>MPLIFKIGYNVIPLQDVILPTPSSKVLKYLIQSGKLIPSLKDLITSRDKYKPIFISHLGFNQRRIFQTNGNLKTITKGSRLSSIIAFSTQANVLSEVADEGIFETVYGKFHIMIESIEIVEVEKLKEEVEKHMNDNIRVRFVSPTLLSSKVLLPPSLSERYKKIHAGYSTLPSVGLIVAYAYNVYCNLIGKKE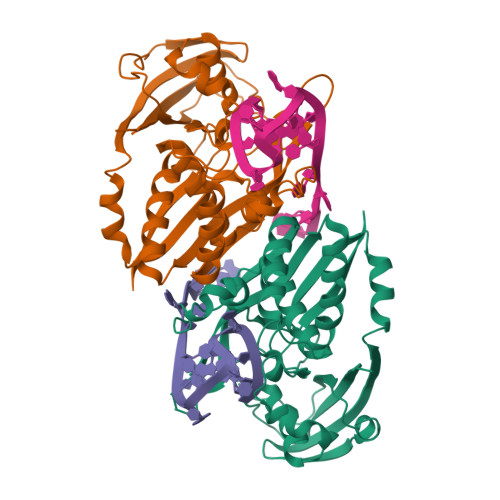VEVRAFKFGILSNALSRIIGYDLHPVTVAIGEDSKGNLRKARGVMGWIEFDIPDERLKRRALNYLLTSSYLGIGRSRGIGFGEIRLEFRKIEEKEG[8x]>[4x]AT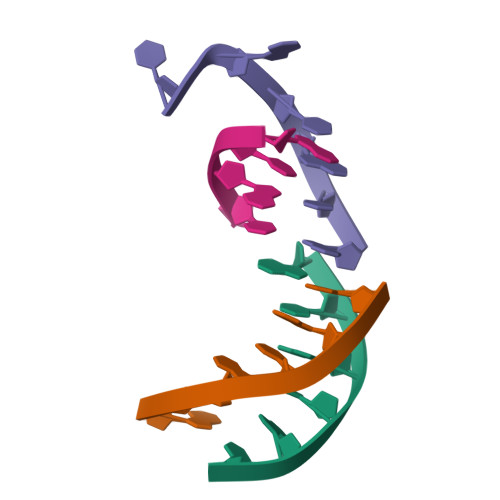ATAT> GPMDGTAAEPRPGAGSLQHAQPPPQPRKKRPEDFKFGKILGEGSFSTVVLARELATSREYAIKILEKRHIIKENKVPYVTRERDVMSRLDHPFFVKLYFTFQDDEKLYFGLSYAKNGCLLKYIRKIGSFDETCTRFYTAEIVSALEYLHGKGIIHRDLKPENILLNEDMHIQITDFGTAKVLSPESKQARANSFVGTAQYVSPELLTEKSASKSSDLWALGCIIYQLVAGLPPFRAGNEYLIFQKIIKLEYDFPEKFFPKARDLVEKLLVLDATKRLGCEEMEGYGPLKAHPFFESVTWENLHQQ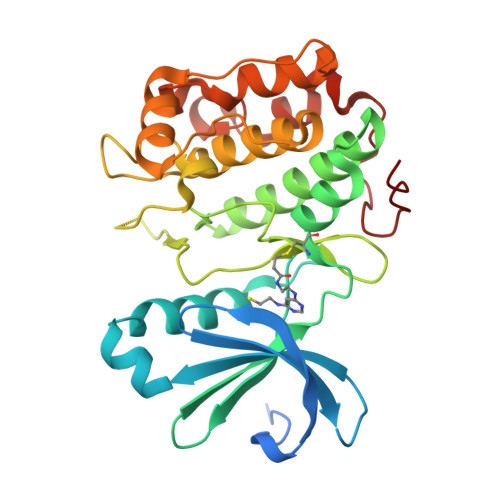TPPKLT> TENLDNVALSSSPIHSGFLVSFMVDARGGAMRGCRHNGLRIIIPPRK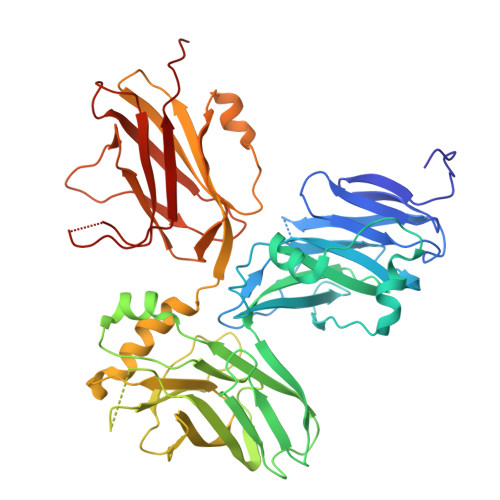CTAPTRVTCRLVKRHRLATMPPMVEGEGLASRLIEVGPSGAQFLGPVIVEIPHFAALRGKERELVVLRSENGDSWKEHFCDYTEDELNEILNGMDEVLDSPEDLEKKRICRIITRDFPQYFAVVSRIKQDSNLIGPEGGVLSSTVVPQVQAVFPEGALTKRIRVGLQAQPMHSELVKKILGNKATFSPIVTLEPRRRKFHKPITMTIPVPKASSDVMLNGFGGDAPTLRLLCSITGGTTPAQWEDITGTTPLTFVNECVSFTTNVSARFWLIDCRQIQESVTFASQVYREIICVPYMAKFVVFAKSHDPIEARLRCFCMTDDKVDKTLEQQENFAEVARSRDVEVLEGKPIYVDCFGNLVPLTKSGQHHIFSFFAFKENRLPLFVKVRDTTQEPCGRLSFMKEPKSTRGLVHQAICNLNITLPIYTKE> HHHHHHMQHLVLIGFMGSGKSSLAQELGLALKLEVLDTDMIISERVGLSVREIFEELGEDNFAMFEKNLIDELKTLKTPHVISTGGGIVMHENLKGLGTTFYLKMDFETLIKRLNQKEREKRP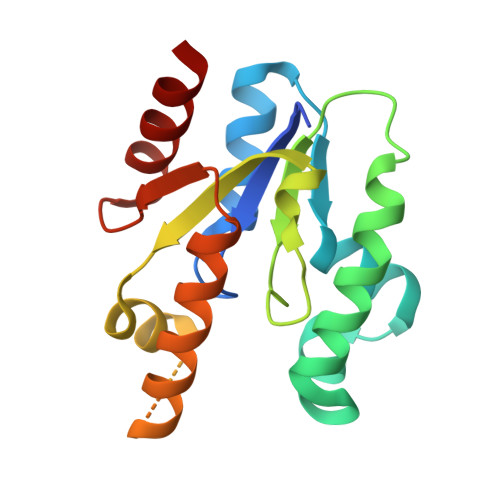LLNNLTQAKELFEKRQALYEKNASFIIDARGGLNNSLKQVLQFIA>[2x]MGVDPFERNKILGRGINIGNALEAPNEGDWGVVIKDEFFDIIKEAGFSHVRIPIRWSTHAYAFPPYKIMDRFFKRVDEVINGALKRGLAVVINIHHYEELMNDPEEHKERFLALWKQIADRYKDYPETLFFEILNAPHGNLTPEKWNELLEEALKVIRSID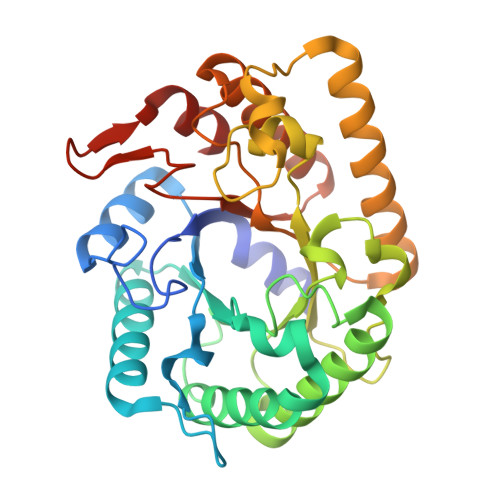KKHTIIIGTAEWGGISALEKLSVPKWEKNSIVTIHYYNPFEFTHQGAEWVEGSEKWLGRKWGSPDDQKHLIEEFNFIEEWSKKNKRPIYIGEFGAYRKADLESRIKWTSFVVREMEKRRWSLAYWEFCSGFGVYDTLRKTWNKDLLEALIGGDSIE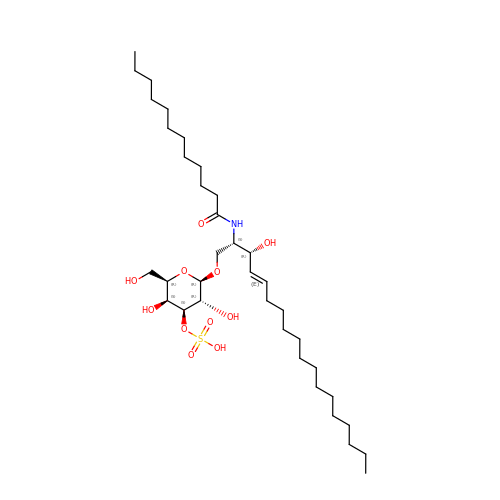N-{(2S,3R,4E)-3-hydroxy-1-[(3-O-sulfo-beta-D-galactopyranosyl)oxy]octadec-4-en-2-yl}dodecanamide | C36 H69 N O11 S | FWVDYZZBQLRRDU-AZNTWQPMSA-N>GPSHMATTLIVARLKPGDHRDQISRLFAESDTTELPDLVGVQERRLLTFKDLYFHLVRTDEALSKTLTPQHD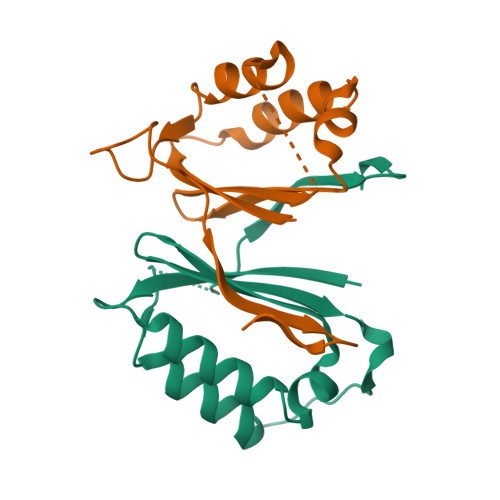HPLFRSISEAMDEYVTPYEGAWGSVEQASARQFYHWKRGLGRVQP[2x]(1-HYDROXYNONANE-1,1-DIYL)BIS(PHOSPHONIC 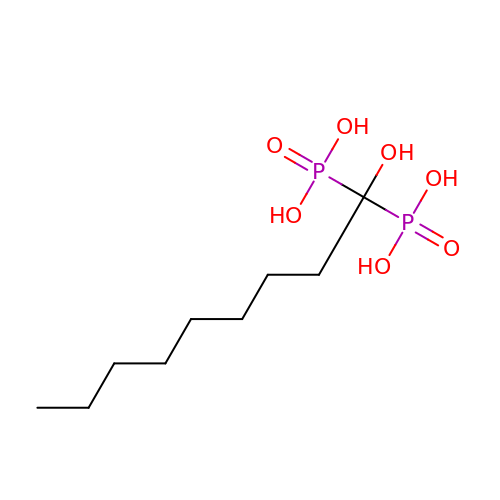ACID) | C9 H22 O7 P2 | COHUUYPEYRMWTH-UHFFFAOYSA-N> ADAPGDDYVISAPEGMKAKPKGDKPGALQKTVPFPHSKHATVECAQCHHTLEADGGAVKKCTTSGCHDSLEFRDKANAKDIKLVE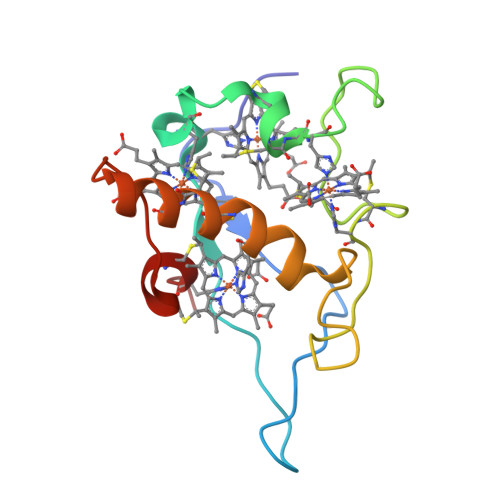NAYHTQCIDCHKALKKDKKPTGPTACGKCHTTN>[5x]DPFTMLQIEFITDLGARVTVNVEHESRLLDVQRHYGRLGWTSGEIPSGGYQFPIENEADFDWSLIGARKWKSPEGEELVIHRGHAYRRRELEAVDSRKLKLPAAIKYSRGAKVSDPQHVREKADGDIEYVSLAIFRGGKRQERYAVPG

Owing to its abundance in the cell post-IR, its ability to bind ssDNA in vitro and a disordered C-terminus, DdrB has been implicated as a stress-inducible functional equivalent to canonical single-stranded binding protein (SSB). The crystal structure of DdrB confirmed that in addition to be being functionally dissimilar to canonical SSB, DdrB is structurally distinct and likely does not bind ssDNA in the same way as SSB, as it lacks an OB-fold. SSA appears to function independently of RecA and is thought to play a role early during DSB repair in Deinococcus spp., particularly when the number of strand breakages is extensive. It has been suggested that DdrB may play an important role in SSA due to its ssDNA annealing activity, similar to Rad52 in the analogous eukaryotic pathway.

We report the X-ray structure of DdrB in complex with ssDNA to 2.3 Å and assessed the DNA binding activity of a number of point mutants generated based on this structure by fluorescence polarization. Molecular replacement produced a good quality electron density map for the entire asymmetric unit (one DdrBDr pentamer) with very clear density for bound ssDNA in two clefts formed between three DdrB subunits. The coordinates for this model have been deposited with two individual 4-mers of dT bound between subunits E/A (T1–T4) and A/B (T5–T8); however, when crystallographic symmetry is applied, the two 4-mers form a continuous 8-mer related by the symmetry operation [−Y, X–Y, Z + 2/3]. Although there are five channels formed between adjacent monomers within a single pentamer, only two are occupied by DNA. The regions joining β6–β7 and β7–β8 (Lβ7–β8), which were unstructured in the apo model, are stabilized through interactions with ssDNA and are now visible in the electron density. The β6′–β7′ hairpin is involved in direct interactions with ssDNA in the DNA-bound structure, as well as playing a key role in mediating the oligomeric assembly observed within the crystal lattice. Overall, the interactions between DdrB and the bound ssDNA consist largely of charged interactions with the phosphate backbone, and interactions with the planar surfaces of the nucleobases. W66 in particular is involved in stabilizing three nucleobases (T3, T6 and T7) through both face–face and T-shaped π–π interactions. Interaction with the continuous 8-mer is coordinated by two pentamers that form an extensive protein–protein interface stabilized by numerous electrostatic and hydrogen bonding interactions, and significant buried surface area (1082 Å2 as calculated by the PISA server). Dimerization of DdrB pentamers is therefore required to generate the DNA binding channel occupied within the crystal structure.> MHHHHHHMLEAKFEEASLFKRIIDGFKDCVQLVNFQCKEDGIIAQAVDDSRVLLVSLEIGVEAFQEYRCDHPVTLG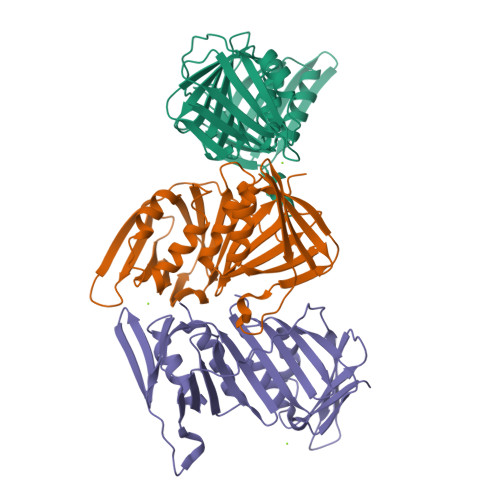MDLTSLSKILRCGNNTDTLTLIADNTPDSIILLFEDTKKDRIAEYSLKLMDIDADFAKAEELQYDSTLSLPSSEFSKIVRDLSQLSDSINIMITKETIKFVADGDIGSGSVIIKPFVDMEHPETSIKLEMDQPVDLTFGAKYLLDIIKGSSLSDRVGIRLSSEAPALFQFDLKSGFLQFFLAPKFNDEE>MSTRKAVIGYYFIPTNQINNYTETDTSVVPFPVSNITPAKAKQLTHINFSFLDINSNLECAWDPATNDAKARDVVNRLTALKAHNPSLRIMFSIGGWYYSNDLGVSHANYVNAVKTPASRAKFAQSCVRIMKDYGFDGVDINWEYPQAAEVDGFIAALQEIRTLLNQQTITDGRQALPYQLTIAGAGGAFFLSRYYSKLAQIVAPLDYINLMTYDLAGPWEKVTNHQAALFGDAAGPTFYNALREANLGWSWEELTRAFPSPFSLTVDAAVQQHLMMEGVPSAKIVMGVPFYGRAFKGVSGGNGGQYSSHSTPGEDPYPS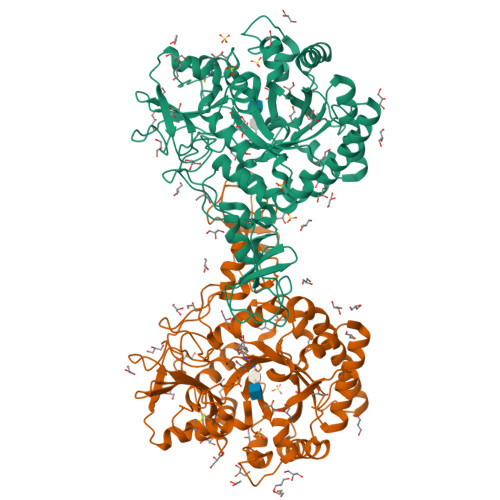TDYWLVGCEECVRDKDPRIASYRQLEQMLQGNYGYQRLWNDKTKTPYLYHAQNGLFVTYDDAESFKYKAKYIKQQQLGGVMFWHLGQDNRNGDLLAALDRYFNAADYDDSQLDMGTGLRYTGVGPGNLPIMTAPAYVPGTTYAQGALVSYQGYVWQTKWGYITSAPGSDSAWLKVGRVR[2x]>GSHMSQTEPPEDLMQYEAMAQDALRGVVKAALKKAAAPGGLPEPH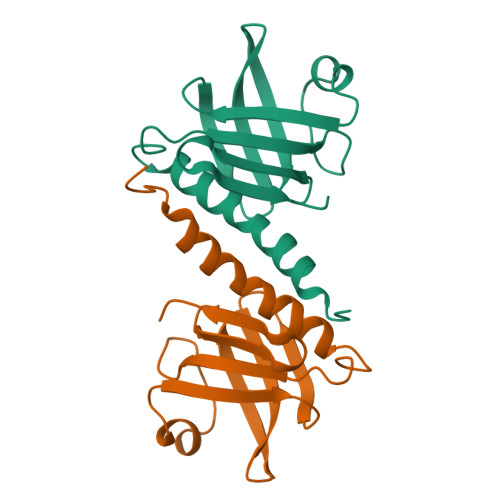HLYITFKTKAAGVSGPQDLLSKYPDEMTIVLQHQYWDLAPGETFFSVTLKFGGQPKRLSVPYAALTRFYDPSVQFALQFSAPE[4x]3-pyrrol-1-ylthiophene-2-carboxylic acid | C9 H7 N O2 S | 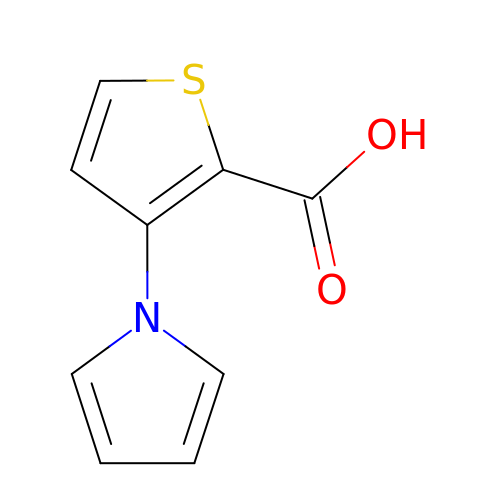WSCYUZJLJQNLSQ-UHFFFAOYSA-N> GMITIENSKFKAGIAERGAELQSLVNKADNYEYVWTGDKTFWNRHAPILFPSIGKSNQDQYRLGAKTYPMSQHGFARDYDFDVSDKSDSAVTFTQHQNAETLKKFPFEYTLAVTYMLTDGGLSVHYTVTNDDSKSMPFAL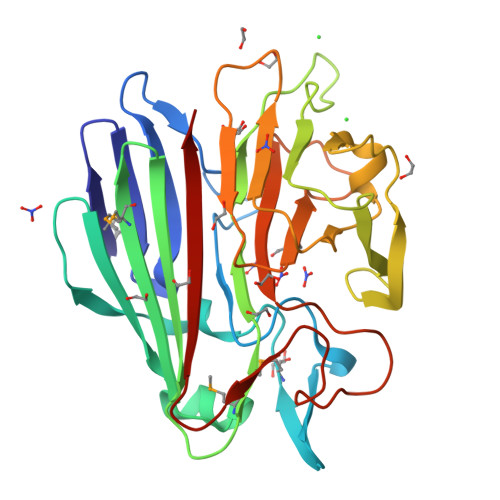GFHPAFNVGLKADGSFDDYDLTVEPLNSPLQRFGIGPVPFRNGDVEDIPGAEGNRLPLTHDLLDGGLVILANSEIAKATLASPHHDHSITLDISDFPYLTIWSPEHKKAPFIAVEPFDGLPDQAGEPTDWYTKLGNTTLSAGANKQLALKVELH>[4x]MSQQPGVLPENMKRYMGRDAQRMNILAGRI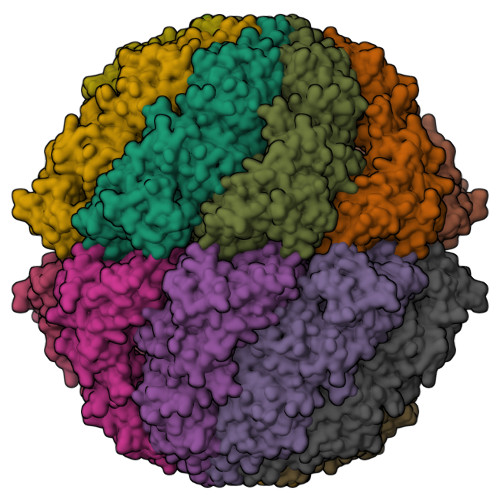IAETVRSTLGPKGMDKMLVDDLGDVVVTNDGVTILREMSVEHPAAKMLIEVAKTQEKEVGDGTTTAVVVAGELLRKAEELLDQNVHPTIVVKGYQAAAQKAQELLKTIACEVGAQDKEILTKIAMTSITGKGAEKAKEKLAEIIVEAVSAVVDDEGKVDKDLIKIEKKSGASIDDTELIKGVLVDKERVSAQMPKKVTDAKIALLNCAIEIKETETDAEIRITDPAKLMEFIEQEEKMLKDMVAEIKASGANVLFCQKGIDDLAQHYLAKEGIVAARRVKKSDMEKLAKATGANVITNIKDLSAQDLGDAGLVEERKISGDSMIFVEECKHPKAVTMLIRGTTEHVIEEVARAVDDAVGVVGCTIEDGRIVSGGGSTEVELSMKLREYAEGISGREQLAVRAFADALEVIPRTLAENAGLDAIEILVKVRAAHASNGNKCAGLNVFTGAVEDMCENGVVEPLRVKTQAIQSAAESTEMLLRIDDVIAAEKLRGAPDMGDMGGMPGMGGMPGMM> VHQVLYRALVSTKWLAESVRAGKVGPGLRVLDASWYSPGTREAR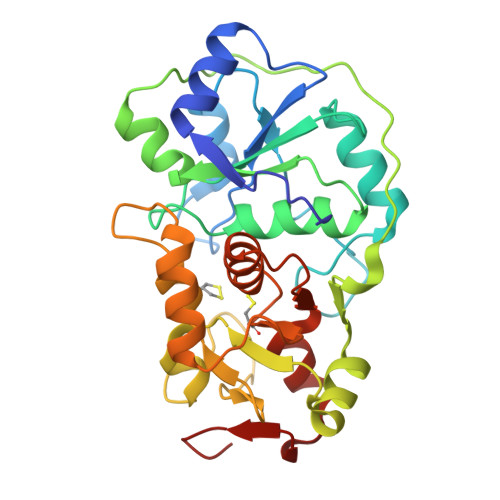KEYLERHVPGASFFDIEECRDKASPYEVMLPSEAGFADYVGSLGISNDTHVVVYDGDDLGSFYAPRVWWMFRVFGHRTVSVLNGGFRNWLKEGHPVTSEPSRPEPAIFKATLNRSLLKTYEQVLENLESKRFQLVDSRAQGRYLGTQPEPDAVGLDSGHIRGSVNMPFMNFLTEDGFEKSPEELRAMFEAKKVDLTKPLIATCRKGVTACHIALAAYLCGKPDVAIYDGSWFEWFHRAPPETWVSQGKG>MAITADDIAVQYPIPTYRFIVTLGDEQVPFTSASGLDINFDTIEYRDGTGNWFKMPGQRQAPNITLSKGVFPGKNAMYEWINAIQLNQVEKKDIMISLTNEAGTEVLVSWNVSNAFPTSLTSPSFDATSNEIAVQQITLMADRVTIQTA[2x];> MTVTTTYPGVYLSEDAVSSFSVNSAATAVPLFAYDSENTNTINKPIQVFRNWAEFTVEYPTPLEDAFYTSLSLWFMHGGGKCYLVNEANIADAVAQYDDITLIVAAGTDTTTYTAFTTVVGQGYRIFGLFDGPKEKIAGTAKPDEVMEEYPTSPFGAVFYPWGTLASGAAVPPSAIAAASITQTDRTRGVWKAPANQAVNGVTPAFAVSDDFQGKYNQGKALNMIRTFSGQGTVVWGARTLEDSDNWRYIPVRRLFNAVERDIQKSLNKLVFEPNSQPTWQRVKAAVDSYLHSLWQQGALAGNTPADAWFVQVGKDLTMTQEEINQGKMIIKIGLAAVRPAEFIILQFSQDIAQ;> MATVTSVPGVYIEEDASPAMSVSASATAVPLFVARFTPLKPELAGVITRIGSWLDYTILFDSNVPSSARVTVSSTAVEPSPEFDALETASSKATTTYTYQIDDTEVVDPTASVALRLYFQNGGGPCYLYPLEKADDNGPLAALPDLIDEVGEITLLASPDPDETYRTAVYGALAASLDQHKGYFLLADSVNGDAPSAVGGSAQVAVYYPNVEVPHTRKLDDAEVAIDGYLDDEGKAVTTLAALRVVNTEFAGEIAQSLSGDLSAPLSLPPSALIAGVYGKTDGERGVWKAPANVVLNGVSDVSVRVTNEQQAELNPKGINVIRHFSDRGLVVWGSRTQKDDDDWRYIPVRRLFDAAERDIKKALQPMVFEPNSQLTWKRVQTAIDNYLYRLWQQGALAGNKAEEAYFVRVGKGITMTQDEINQGKMIIQVGMAAVRPAEFIILKFTQDMSQ;> MTMVLPGVSYNETLLTQASNDDPVTMPLFIGYTPPDTAIPVTVMQPVSVGSLTQANSLFGQRGTLAYSLRHFFENGGLQCYVLPLGPGKGEPAARLQELIAALQTPQMLETLLADDKTGLVLVPELSELNEVSSTSLSAEGVDAAEVDADALWYQGWQVLLTLCRQAPQRFALLELPEDPASAVTLTQQSFSADQCQRGAAWWPRLETSYQDESSAPVVLSPLPAVAAAIQRSAHDNGVWKAPANIALAKTRRPTQSILTSQALLDNQGVSCNLIRSFVGKGVRLWGCRTLLNEENTAWRYIQIRLLVSSVEHYLSKLARAYLFEPNTAPTWMKLKGQVWTWLRQQWLAGAFFGTVEDEAFSLSIGLDETMTEDDIRHGKMILQVRLALLAPAEFIAISLTLDLRDGTASAQTGGQS;> MSTPAVSHRFLVNFLFNNIPNPFDIAFQRISGLSRTLEVSQHREGGENVRNLWLAEQVNHGSLVLERGVMNASPLTLQFDRVLRRESTQWANVVIMLLNELSLPVTTWTLSHALPVRWQMGDLDAGSNQVLINTLELRYQDMRMLGVKL;> MSLLERGLSKLTLNAWKDREGKIPAGSMSAMYNPETIQLDYQTRFDTEDTINTASQSNRYVISEPVGLNLTLLFDSQMPGNTTPIETQLAMLKSLCAVDAATGSPYFLRITWGKMRWENKGWFAGRARDLSVTYTLFDRDATPLRATVQLSLVADESFVIQQSLKTQSAPDRALVSVPDLASLPLLALSAGGVLASSVDYLSLAWDNDLDNLDDFQTGDFLRATKGEEV;> MSNDILKATLGQCWAFPPRFSPDTGVSLTAGVEAVMQSLRVLFMTEPGERIMRESYGGGMHDFIFENITDELLANIHNRIEESILRHEPRALLKDVIIQPDKQEASRLRAQITVYLAGSDLVETVDGTLNIHDGQTLRLL;> MSDLEQLKQILGNGLTDQTFLLEPRTGKGLLNLMAKYTEAVPFAGHTDADWKDFWMAGCTLEALSDIYQYPGLAEKKLPVQQAFLLALLHLLETPRAMLNTVPARHRSLYYRDLLGFAPRAPQPDSVAVSFTLQRNSSPYALPAGSLLDGGQDSAGNSITYQTDDSLLITGQQLEQLCWTAQVGETWKRYTAIDSATGVTLPAEGLRLFTATGQGTDTKEKAPELYLGFSGTSAQDTLSLYWSVRASSALDVTWWYYQGTKWASLDAELQDNTASLSVSNLWRARLPADSQPGSGLPQDDEPLEAGYYWIKGTLKENKEAKDENSPAEAMPQLQAVLANAMTATLNVAQAIDDSHFSQPLPANTINQLVTPVAAISDVRQPLPSVGGQPRETEMAMLQRAAPRIAHRQRAITWNNMRSLLMEHYPEIFDVRFPDVDKLSRLPALEVQSLMVIPDGRYGDNDDALRPALSNGRLSRMAQWLSQYTSLWAAPTLKNPKYIDVTARYRVTFVVGIRPDYGYRQLAAQLQHDYMPWATDRRQAVTPGNQVDYYQLLATLQQSPLVQSVNALVLSHDVIDETGKPTSMETQSTVTARDDEVLILCPEGETHV;> MSKENALFPAVKDAIVFDALWQQAHEKVTALSGEIWTDTGDHDPGVTLLQSATWNCSDLSYRASLSLNDLLTHQDQSTLFPEEFGPEQVLTCNTVTAEDYRRALLDVHSSDIQALDTPEQDFLFSDVSLTQEPKEHRFHWWYNAEKREYSFRKPTDSGEVNELKLRGNLWLSLVPTRYTQSLSPENLAAVEQCLAEFLAAHRNLGEVVSRITWLQPATFSPRMTIELADNIGDINQVAAQIYQVTDAFLRPAVARYTTEQRRALGDADDAIFEGPRLKHGWQQTAPSQITSGGYVLNLGPLVNLLLAIPGVASLSTLSVDKGDGHITAVTGDNLRWQVADGYYPLLWGAPPLSLLAGDDSPLTLVSKGGIRNTLESEAMAGYLTQADLIVTTPTVLPAGRFRDQTLYIPIGQRQPECYALQQPDTVIDDQTRAVHQFLLPVDQLLADGTAELAQLPTLLAFKNRGDAIRGTRWPYTNAMVQQAIHQPYAKTLEAIAQQDAAIFTQDKQPVGGNYARELDFLQYLLGYFGTQRAALPLTLDLPDFLATQRAYLAQQPALGYDRINIRIDQVSALQKRIAARIGLDSICFADNPDLGQLPFYLIEHRQLLPQTPDSTFDSEQTPSGFAVAEPDITLTQAGSVGKVVQGQLIDLIAIEGGSRLHVSRLLVIKAEGDSFTVSTENSQQLHNTLSRLETAWASHNLRWQNSNVWLQDMDYRLNYAEAKLQPANPQQRLLASNAQSPYPAMVSVGDG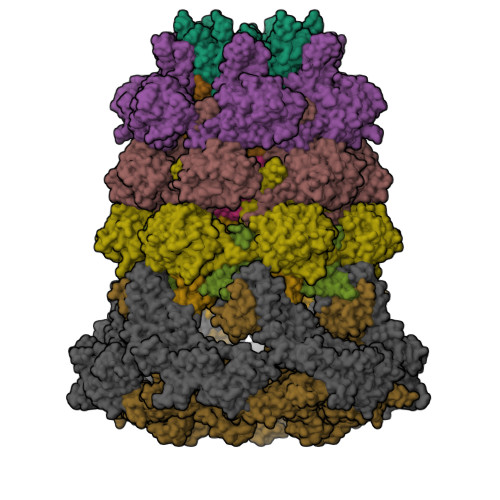IVLRPAGLQFYMPGANATRAATLDADWQLAATVKAVDPIAGTLLIEKAAGSTEDFPSAESSFRYQWAFSQANYATTDRFSFVVSAVLNRRLIENPNIVPEQLVAWIQETIMAEFPAHVSLINHWLDDATFNNFGVTYSRWQNSGMPLGDDAFALMQILTLGHLPVTQLDIGLMRIATEEQRTEVIGDGSQWHEDVILREELFYVPKDVQTTL>[6x]MLDSKLKAPVFTVRTQGREYGEFVLEPLERGFGVTLGNPLRRILLSSIPGTAVTSVYIEDVLHEFSTIPGVKEDVVEIILNLKELVVRFLNPSLQTVTLLLKAEGPKEVKARDFLPVADVEIMNPDLHIATLEEGGRLNMEVRVDRGVGYVPAEKHGIKDRINAIPVDAVFSPVRRVAFQVEDTRLGQRTDLDKLTLRIWTDGSVTPLEALNQAVEILREHLTYFSNPQAAAVAAPEEAKEPEAPPEQEEELDLPLEELGLSTRVLHSLKEEGIESVRALLALNLKDLKNIPGIGERSLEEIKEALEKKGFTLKE;>[3x]MEIKRFGRIREVIPLPPLTEIQVESYRRALQADVPPEKRENVGIQAAFRETFPIEEEDKGKGGLVLDFLEYRLGEPPFPQDECREKDLTYQAPLYARLQLIHKDTG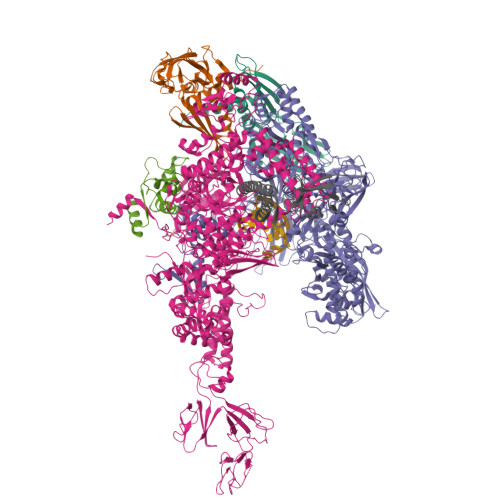LIKEDEVFLGHIPLMTEDGSFIINGADRVIVSQIHRSPGVYFTPDPARPGRYIASIIPLPKRGPWIDLEVEPNGVVSMKVNKRKFPLVLLLRVLGYDQETLARELGAYGELVQGLMDESVFAMRPEEALIRLFTLLRPGDPPKRDKAVAYVYGLIADPRRYDLGEAGRYKAEEKLGIRLSGRTLARFEDGEFKDEVFLPTLRYLFALTAGVPGHEVDDIDHLGNRRIRTVGELMTDQFRVGLARLARGVRERMLMGSEDSLTPAKLVNSRPLEAAIREFFSRSQLSQFKDETNPLSSLRHKRRISALGPGGLTRERAGFDVRDVHRTHYGRICPVETPEGANIGLITSLAAYARVDELGFIRTPYRRVVGGVVTDEVVYMTATEEDRYTIAQANTPLEGNRIAAERVVARRKGEPVIVSPEEVEFMDVSPKQVFSVNTNLIPFLEHDDANRALMGSNMQTQAVPLIRAQAPVVMTGLEERVVRDSLAALYAEEDGEVAKVDGNRIVVRYEDGRLVEYPLRRFYRSNQGTALDQRPRVVVGQRVRKGDLLADGPASENGFLALGQNVLVAIMPFDGYNFEDAIVISEELLKRDFYTSIHIERYEIEARDTKLGPERITRDIPHLSEAALRDLDEEGVVRIGAEVKPGDILVGRTSFKGESEPTPEERLLRSIFGEKARDVKDTSLRVPPGEGGIVVRTVRLRRGDPGVELKPGVREVVRVYVAQKRKLQVGDKLANRHGNKGVVAKILPVEDMPHLPDGTPVDVILNPLGVPSRMNLGQILETHLGLAGYFLGQRYISPIFDGAKEPEIKELLAQAFEVYFGKRKGEGFGVDKREVEVLRRAEKLGLVTPGKTPEEQLKELFLQGKVVLYDGRTGEPIEGPIVVGQMFIMKLYHMVEDKMHARSTGPYSLITQQPLGGKAQFGGQRFGEMEVWALEAYGAAHTLQEMLTLKSDDIEGRNAAYEAIIKGEDVPEPSVPESFRVLVKELQALALDVQTLDEKDNPVDIFEGLASKR;>MKKEVRKVRIALASPEKIRSWSYGEVEKPETINYRTLKPERDGLFDERIFGPIKDYECACGKYKRQRFEGKVCERCGVEVTKSIVRRYRMGHIELATPAAHIWFVKDVPSKIGTLLDLSATELEQVLYFSKYIVLDPKGAILNGVPVEKRQLLTDEEYRELRYGKQETYPLPPGVDALVKDGEEVVKGQELAPGVVSRLDGVALYRFPRRVRVEYVKKERAGLRLPLAAWVEKEAYKPGEILAELPEPYLFRAEEEGVVELKELEEGAFLVLRREDEPVATYFLPVGMTPLVVHGEIVEKGQPLAEAKGLLRMPRQVRAAQVEAEEEGETVYLTLFLEWTEPKDYRVQPHMNVVVPEGARVEAGDKIVAAIDPEEEVIAEAEGVVHLHEPASILVVKARVYPFEDDVEVSTGDRVAPGDVLADGGKVKSDVYGRVEVDLVRNVVRVVESYDIDARMGAEAIQQLLKELDLEALEKELLEEMKHPSRARRAKARKRLEVVRAFLDSGNRPEWMILEAVPVLPPDLRPMVQVDGGRFATSDLNDLYRRLINRNNRLKKLLAQGAPEIIIRNEKRMLQEAVDALLDNGRRGAPVTNPGSDRPLRSLTDILSGKQGRFRQNLLGKRVDYSGRSVIVVGPQLKLHQCGLPKRMALELFKPFLLKKMEEKGIAPNVKAARRMLERQRDIKDEVWDALEEVIHGKVVLLNRAPTLHRLGIQAFQPVLVEGQSIQLHPLVCEAFNADFDGDQMAVHVPLSSFAQAEARIQMLSAHNLLSPASGEPLAKPSRDIILGLYYITQVRKEKKGAGLEFATPEEALAAHERGEVALNAPIKVAGRETSVGRLKYVFANPDEALLAVAHGIVDLQDVVTVRYMGKRLETSPGRILFARIVAEAVEDEKVAWELIQLDVPQEKNSLKDLVYQAFLRLGMEKTARLLDALKYYGFTFSTTSGITIGIDDAVIPEEKKQYLEEADRKLLQIEQAYEMGFLTDRERYDQILQLWTETTEKVTQAVFKNFEENYPFNPLYVMAQSGARGNPQQIRQLCGLRGLMQKPSGETFEVPVRSSFREGLTVLEYFISSHGARKGGADTALRTADSGYLTRKLVDVTHEIVVREADCGTTNYISVPLFQPDEVTRSLRLRKRADIEAGLYGRVLAREVEVLGVRLEEGRYLSMDDVHLLIKAAEAGEIQEVPVRSPLTCQTRYGVCQKCYGYDLSMARPVSIGEAVGIVAAQSIGEPGTQLTMRTFHTGGVAGAADITQGLPRVIELFEARRPKAKAVISEIDGVVRIEETEEKLSVFVESEGFSKEYKLPKEARLLVKDGDYVEAGQPLTRGAIDPHQLLEAKGPEAVERYLVEEIQKVYRAQGVKLHDKHIEIVVRQMMKYVEVTDPGDSRLLEGQVLEKWDVEALNERLIAEGKTPVAWKPLLMGVTKSALSTKSWLSAASFQNTTHVLTEAAIAGKKDELIGLKENVILGRLIPAGTGSDFVRFTQVVDQKTLKAIEEARKEAVEAKERPAARRGVKREQPGKQA[3x];>MAEPGIDKLFGMVDSKYRLTVVVAKRAQQLLRHGFKNTVLEPEERPKMQTLEGLFDDPNAVTWAMKELLTGRLVFGENLVPEDRLQKEMERLYPVEREE[3x];>MAREVKLTKAGYERLMQQLERERERLQEATKILQELMESSDDYDDSGLEAAKQEKARIEARIDSLEDILSRAVILEEGSGEVIGLGSVVELEDPLSGERLSVQVVSPAEANVLDTPMKISDASPMGKALLGHRVGDVLSLDTPKGRREFRVVAIHG[3x]> MTLQQVSTQAITSDERRFAYAVL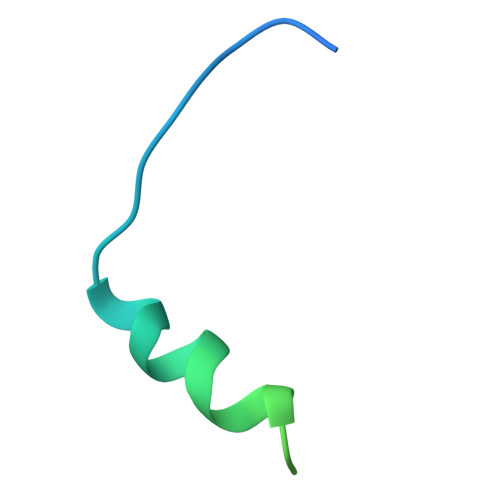EHAKNTILNRQDVAKLLPRASNFELSQHHHHHH> MKEFYLTVEQIGDSIFERYIDSNGRERTREVEYKPSLFAHCPESQATKYFDIYGKPCTRKLFANMRDASQWIKRMEDIGLEALGMDDFKLAYLSDTYNYEIKYDHTKIRVANFDIEVTSPDGFPEPSQAKHPIDAITHYDSIDDRFYVFDLLNSPYGNVEEWSIEIAAKLQEQGGDEVPSEIIDKIIYMPFDNEKELLMEYLNFWQQKTPVILTGWNVESFAIPYVYNRIKNIFGESTAKRLSPHRKTRVKVIENMYGSREIITLFGISVLDYIDLYKKFSFTNQPSYSLDYISEFELNVGKLKYDGPISKLRESNHQRYISYNIIAVYRVLQIDAKRQFINLSLDMGYYAKIQIQSVFSPIKTWDAIIFNSLKEQNKVIPQGRSHPVQPYPGAFVKEPIPNRYKYVMSFDLTSAYPSIIRQVNISPETIAGTFKVAPLHDYINAVAERPSDVYSCSPNGMMYYKDRDGVVPTEITKVFNQRKEHKGYMLAAQRNGEIIKEALHNPNLSVDEPLDVDYRFDFSDEIKEKIKKLSAKSLNEMLFRAQRTEVAGMTAQINRKLLINSLYGALGNVWFRYYDLRNATAITTFGQMALQWIERKVNEYLNEVCGTEGEAFVLYGDTDSIYVSADKIIDKVGESKFRDTNHWVDFLDKFARERMEPAIDRGFREMCEYMNNKQHLMFMDREAIAGPPLGSKGIGGFWTGKKRYALNVWDMEGTRYAEPKLKIMGLETQKSSTPKAVQKALKECIRRMLQEGEESLQEYFKEFEKEFRQLNYISIASVSSANNIAKYDVGGFPGPKCPFHIRGILTYNRAIKGNIDAPQVVEGEKVYVLPLREGNPFGDKCIAWPSGTEITDLIKDDVLHWMDYTVLLEKTFIKPLEGFTSAAKLDYEKKASLFDMF

The replicative DNA pol from bacteriophage RB69 (RB69pol) is a member of the B family and is responsible for DNA synthesis of both leading and lagging strands of its genome. It has extensive sequence similarity to human replicative pols α and δ and therefore has been regarded as a good model for B family pols. Our previous reported 1.8 Å resolution structure of wt RB69pol showed that L415 is located right below the triphosphate tail of the incoming dNTP, where a small hydrophobic cavity exists at the tip of the L415 side chain. To provide a structural basis that could account for the different kinetic behavior observed among L415 variants and wt RB69pol, we determined the crystal structures of three ternary complexes: dTTP/dA-with the L415A mutant; dATP/dT-with the L415G mutant and dATP/dT-with the L415M mutant with resolutions ranging from 1.80 to 2.04 Å and Rfree values ranging from 21.3% to 21.9%.

Replacing L415 with either Ala or Gly greatly enlarges the size of this cavity. In particular, the change of the metal ion A position in both the L415A and L415G ternary complexes are mediated by an alteration in peptide backbone. Therefore, the 0.5 Å downshifting of the metal ion A from its optimal position observed in the wt RB69pol structure would cause misalignment between the 3′-OH and Pα, possibly reducing the rate of phosphodiester bond formation. This could explain why the kpol values for incorporating a correct dNMP by L415A and L415G mutants are 5- to 25-fold lower than the kpol for wt RB69pol. All three mismatches can be modeled perfectly well into the NBP of L415A. The major difference between the two mutants was that the L415A mutant incorporated incorrect dNMPs 5- to 7-fold more efficiently than the L415G mutant. By replacing L415 with either Ala or Gly, the enlarged cavity provides extra space for nearby residues, such as L412 and Y416. Thus, the increased freedom of L412 and Y416 provides this extra flexibility for the incoming dNTP and allows it to adopt non-Watson–Crick geometry with the templating base. In addition, a water molecule is observed in this hydrophobic cavity when L415 is replaced with Ala or Gly. Our tCo-tCnitro FRET assays show that replacement of L415 with Ala or Gly abolished the pol’s ability to differentiate fully complementary P/Ts from P/Ts with a mismatch at the P/T junction.> MGKTYDVNICYA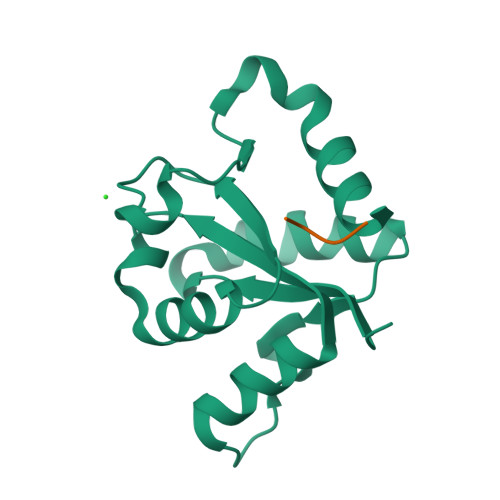PEDREWVINTLVFKLERAGIKTFVNIRDDTPGNFFAENIMDAIENSNRTIVVMSPDFFKNNICDKTLQIGLSHQIIPILYRPCEVPYFLNHMTYLDWCDKDVRPVFWRNLFRDIRNN;> HHHHHH>GHMDSMDHRIERLEYYIQLLVKTVDMDRYPFYALLIDKGLSKEEGEAVMRICDELSEELATQKAQGFVTFDKLLALFAGQLNEKLDVHETIFALYEQGLYQELMEVFIDIMKHFDGS[3x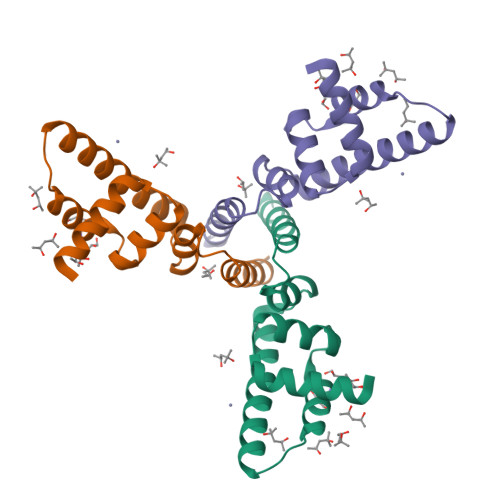]>[2x]QSCATGPRNCKDLLDRGYFLSGWHTIYLPDCRPLTVLCDMDTDGGGWTVFQRR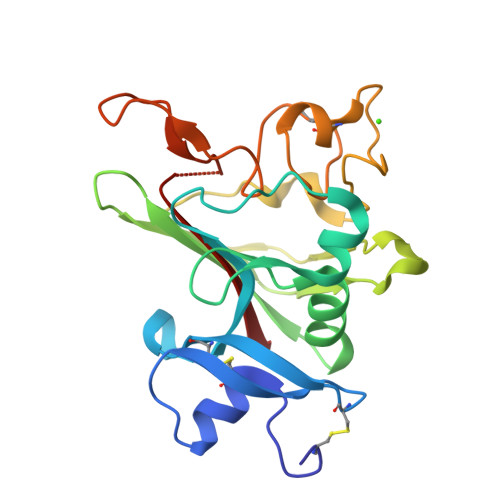MDGSVDFYRDWAAYKQGFGSQLGEFWLGNDNIHALTAQGSSELRTDLVDFEGNHQFAKYKSFKVADEAEKYKLVLGAFVGGSAGNSLTGHNNNFFSTKDQDNDVSSSNCAEKFQGAWWYADCHASNLNGLYLMGPHESYANGINWSAAKGYKYSYKVSEMKVRPA>SNAPVTELTRLKEYMEDQIAKAKESSSLTAQLKFLENAHTEHFVKMGSLTTIYKGGSEVVDRLKIEIRSLYEEMLELKDKCRDQIQQYE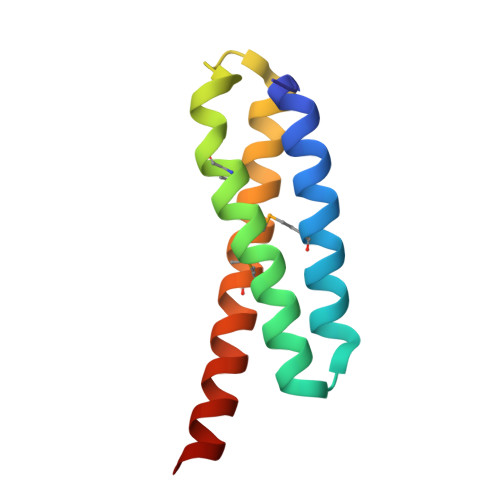TS[2x]>DEITKKYIKDNIINVDDNIIKKKDIFKLKNENN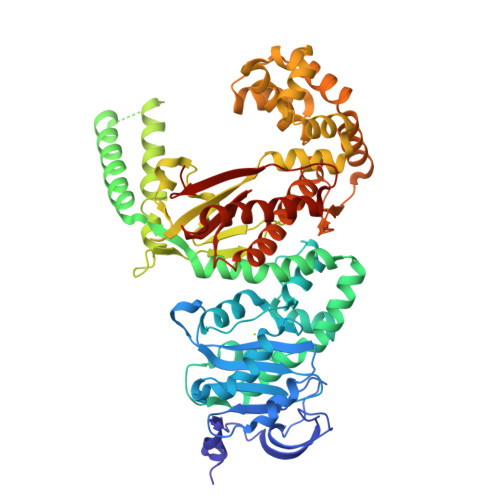EITECAFEYFESKKKFDDDIESRFFIINDNNYNENINLIYKDIKYCGLNIQTTGLEVFDENIRLIQIAVENYPVIIYDMFNINKKDILDGLRKVLENKNIIKIIQNGKFDAKFLLHNNFKIENIFDTYIASKLLDKNKNMYGFKLNNIVEKYLNVILDKQQQNSVWNNSLLNNNQLFYAARDSSCLLKLYKKLKEEIKKENLHIVNDIENKCILPICDMELNGIKVDLENLQKSTNEILNELNIEKDNLKKKLKDENINVNSQQQVLKALQKNNVRDISNKLIENTSDSNLKNFLNHEEIISLRNYRRLYKLYSAFYLKLPLHINTKTNKIHTTFNQLKTFSGRFSSEKPNLQQIPRQKNIREIFIPNDNNIFIIADFKQIELKIAAEITNDEIMLKAYNNNIDLHTLTASIITKKNIPDINKEDRHIAKAINFGLIYGMNYVNLKNYANTYYGLNMSLDQCLYFYNSFFEHYKGIYKWHNQVKQKRALQYSTLSNRKVIFPYFSFTKALNYPVQGTCADILKLALVDLYDNLKDINGKIILCVHDEIIIEVNKKFQEEALKILVQSMENSASYFLKKVKCEVSVKIAENWGSKDLEHHHHH[2x]N-[3-[[3-[2-(4,6-dimethylpyrimidin-2-yl)sulfanylethanoylamino]phenyl]methoxy]phenyl]-1-methyl-pyrazole-4-carboxamide 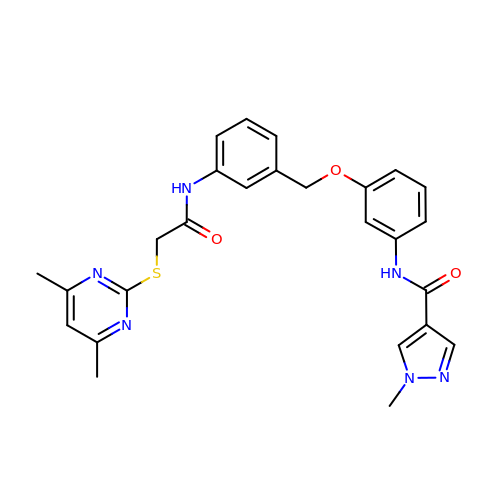| C26 H26 N6 O3 S | SLKIFBBCZNLTHR-UHFFFAOYSA-N> KLPTNLAYERSIDPSDVCFFVVWPDDRKTPLTYNSRTLLGQMEAKSLAYDVSGQPIKSATAEALAQGNPHQVDFCHVPYGASHIECSFSVSFSSELRQPYKCNSSKVKQTLVQLVELYETKIGWTELATRYLMNICNGKWLWKNTRKAYCWNIVLTPWPWNGEKVGFEDIRTNYT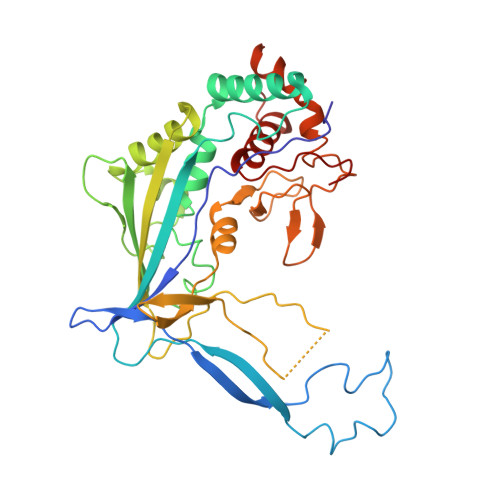SRQDFKNNKNWSAIVEMIKTAFSSTDGLAIFEVRATLHLPTNAMVRPSQVFTEKETQNSRVFQSTTIDGERSPILGAFKTGAAIATIDDWYPEATEPLRVGRFGVHREDVTCYRHPSTGKDFFSILQQAEHYIEVLSANKTPAQETINDMHFLMANLIKGGMFQHKGD> MELADVGAAASSQGVHDQVLPTPNASSRVIVHVDLDCFYAQVEMISNPELKDKPLGVQQKYLVVTCNYEARKLGVKKLMNVRDAKEKCPQLVLVNGEDLTRYREMSYKVTELLEEFSPVVERLGFDENFVDLTEMVEKRLQQLQSDELSAVTVSGHVYNNQSINLLDVLHIRLLVGSQIAAEMREAMYNQLGLTGCAGVASNKLLAKLVSGVFKPNQQTVLLPESCQHLIHSLNHIKEIPGIGYKTAKCL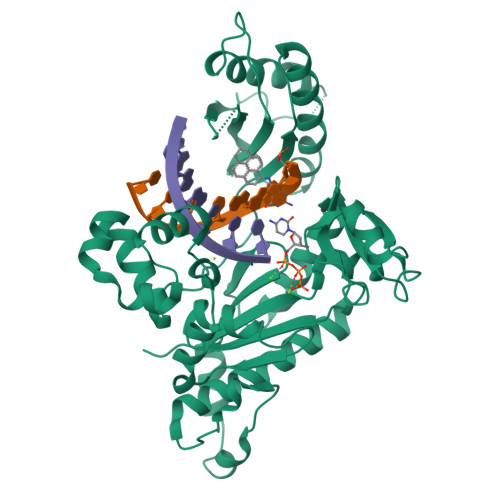EALGINSVRDLQTFSPKILEKELGISVAQRIQKLSFGEDNSPVILSGPPQSFSEEDSFKKCSSEVEAKNKIEELLASLLNRVCQDGRKPHTVRLIIRRYSSEKHYGRESRQCPIPSHVIQKLGTGNYDVMTPMVDILMKLFRNMVNVKMPFHLTLLSVCFCNLKALNTAK>[3x]AWPEEKNYHQPAILNSSALRQIAEGTSISEMWQNDLQPLLIERYPGSPGSYAARQHIMQRIQRLQADWVLEIDTFLSQTPEGERSFSNIISTLNPTAKRHLVLACHYDSKYFSHWNNRVFVGATDSAV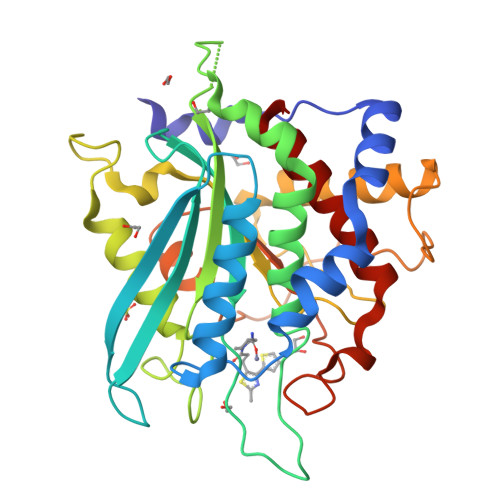PCAMMLELARALDKKLLSLKTVSDSKPDLSLQLIFFDGEEAFLHWSPQDSLYGSRHLAAKMASTPHPPGARGTSQLHGMDLLVLLDLIGAPNPTFPNFFPNSARWFERLQAIEHELHELGLLKDHSLEGRYFQNYSYGGVIQDDHIPFLRRGVPVLHLIPSPFPEVWHTMDDNEENLDESTIDNLNKILQVFVLEYLHL> APAVADKADNAFMMICTALVLFM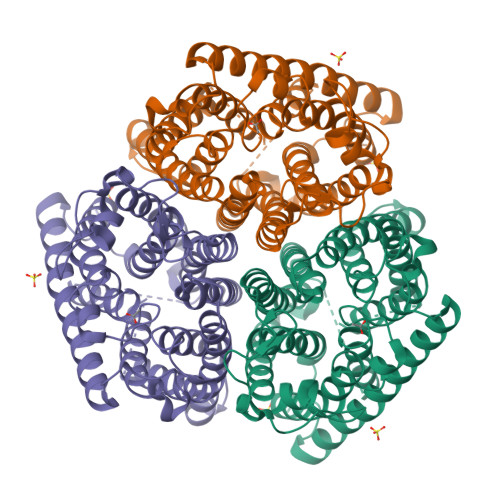TIPGIALFYGGLIRGKNVLSMLTQVTVTFALVCILWVVYGYSLAFGEGNNFFGNINWLMLKNIELTAVMGSIYQYIHVAFQGSFACITVGLIVGALAERIRFSAVLIFVVVWLTLSYIPIAHMVWGGGLLASHGALDFAGGTVVHINAAIAGLVGAYLIGKRVGFGKEAFKPHNLPMVFTGTAILYIGWFGFNAGSAGTANEIAALAFVNTVVATAAAILGWIFGEWALRGKPSLLGACSGAIAGLVGVTPACGYIGVGGALIIGVVAGLAGLWGVTMLKRLLRVDDPCDVFGVHGVCGIVGCIMTGIFAASSLGGVGFAEGVTMGHQLLVQLESIAITIVWSGVVAFIGYKLADLTVGLRVPEEQEREGLDVNSHGENAYNADQAQQPAQADLEHHHHHH>MEERNDWHFNIGAMYEIENVEGYGEDMDGLAEPSVYFNAANGPWRIALAYYQEGPVDYSAGKRGTWFDRPELEVHYQFLE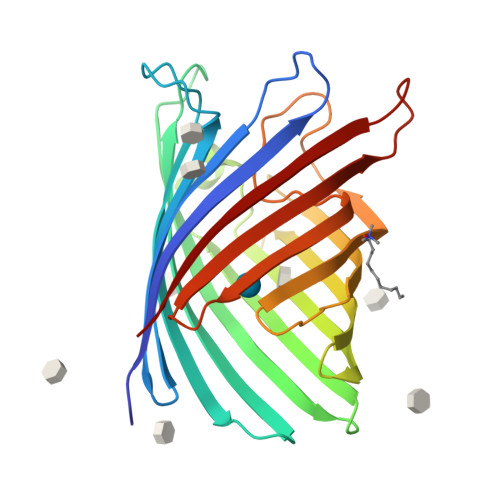NDDFSFGLTGGFRNYGYHYVDEPGKDTANMQRWKIAPDWDVKLTDDLRFNGWLSMYKFANDLNTTGYADTRVETETGLQYTFNETVALRVNYYLERGFNMDDSRNNGEFSTQEIRAYLPLTLGNHSVTPYTRIGLDRWSNWDWQDDIEREGHDFNRVGLFYGYDFQNGLSVSLEYAFEWQDHDEGDSDKFHYAGVGVNYSF[2x]>MRLLNGTPLALALPEAFLYHGASVFTTLRAEGGRPLWLEEHLARLRRHALALGLSYPGDEAFLEDLEALLRAFPKAPCLRLRFTVGEGVRLSEARPYAPLPLSLYREGVRVRLTGYRVHPDLARYKTGNYLPYRLALEEARKEGAFEGLLLDAFGHVVDGSRTSPLLFREGTLYLLEGGLEGITREKVAEAARGLG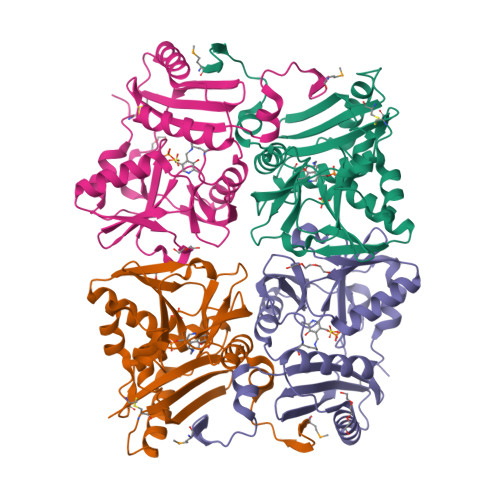LRVERGLFRPEGLRGHLLLAGSGVGLLPVRPPPPELLPLIERFLPACYTE[4x]> GAMVLPNQMVKSMVGKIIRVEMKGEENQLVGKLEGVDDYM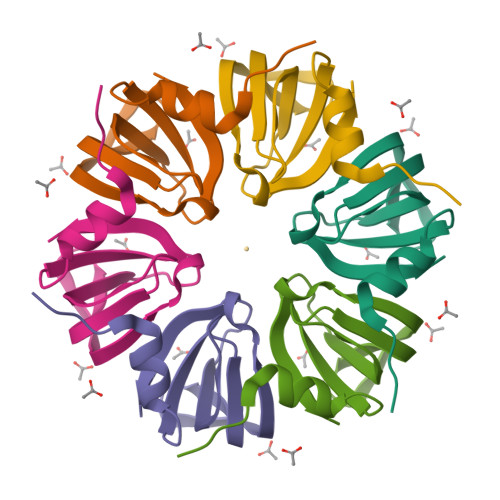NLYLTNAMECKGEEKVRSLGEIVLRGNNVVLIQPQEE> GSHMASMTGGNNMGRMQDEQLELVSGSIGVLKNMSQRIGGELEEQAVMLEDFSHELESTQSRLDNVMKK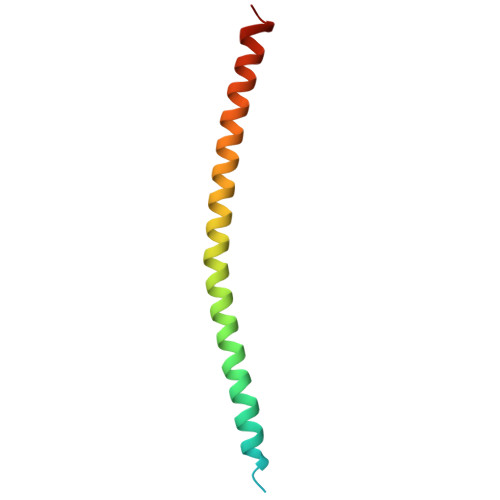LAKVSHMTSDRRQ> NAAIEVEKNNKG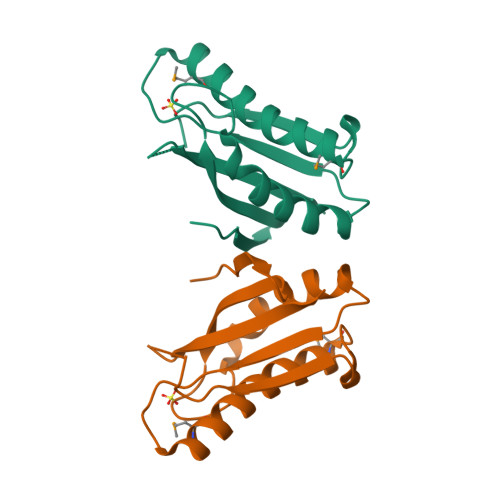INLSFDIEFYPNSFQILQKEYKKIDLIAKLLEKFKKNNILIEGHTEQFGLEEEMHELSEKRARAIGNYLIKMKVKDKDQILFKGWGSQKPKYPKSSPLKAKNRRVEITILN> GMALQEEFIDVNGTRVFQRKMVTDSNRRSIALFHGYSFTSMDWDKADLFNNYSKIGYNVYAPDYPGFGRSASSEKYGIDRGDLKHAAEFIRDYLKANGVARSVIMGASMGGGMVIMTTLQYPDIVDGIIAVAPAWVESLKGDMKKIRQKTLLVWGSKDHVVPIALSKEYASIISGSRLEIVEGSGHPVYIEKPEEFVR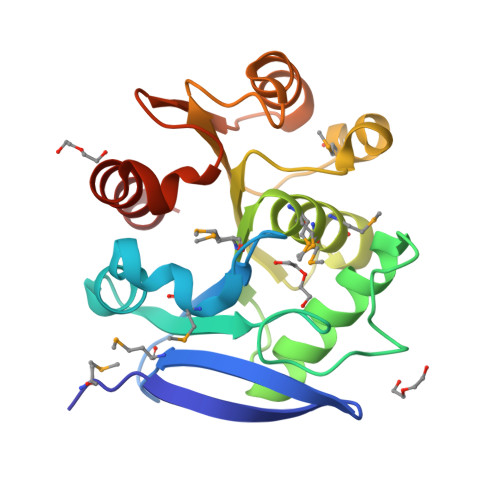ITVDFLRNL>MNIDLKGKVAVVSGGATLIGKAVVQALVSAGAHV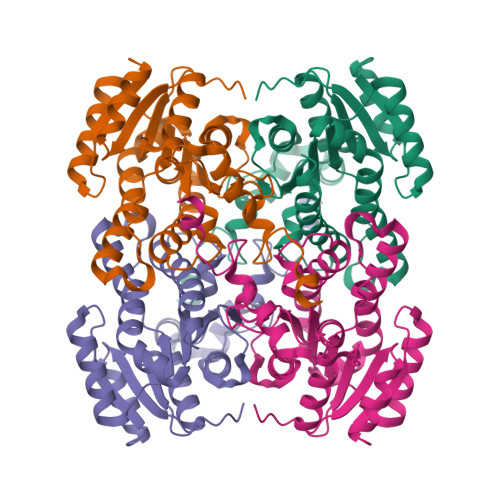AILDIDAKGKAIAESFNHDVMFIQTDLTSDAAIQQAVADIHQHLGEVSYLVNLACTYLDDGFKSSRQDWLQALDINLVSTVELSRALYNDLKKQQGSIVNFTSISAKVAQTGRWLYPVSKAAIRQLTQSMAMDFAADGIRVNSVSPGWTWSRVIAEVSGNNREKADSVAADYHLLGRLGHPEEVANVVLFLLSSAASFVTGADYAVDGGYSVMGPEGLQPAIPRLAE[2x]>MTITPATHAISINPATGEQLSVLPWAGADDIENALQLAAAGFRDWRETNIDYRAEKLRDIGKALRARSEEMAQMITREMGKPINQARAEVAKSANLCDWYAEHGPAMLKAEPTLVENQQAVIEYRPLGTILAIMPWNFPLWQVMRGAVPIILAGNGYLLKHAPNVMGCAQLIAQVFKDAGIPQGVYGWLNADNDGVSQMIKDSRIAAVTVTGSVRAGAAIGAQAGAALKKCVLELGGSDPFIVLNDADLELAVKAAVAGRYQNTGQVCAAAKRFIIEEGIASAFTERFVAAAAALKMGDPRDEENALGPMARFDLRDELHHQVEKTLAQGARLLLGGEKMAGAGNYYPPTVLANVTPEMTAFREEMFGPVAAITIAKDAEHALELANDSEFGLSATIFTTDETQARQMAARLECGGVFINGYCASDARVAFGGVKKSGFGRELSHFGLHEFCNIQTVWKDRI[4x]

The NAD(P)+-dependent succinate semialdehyde dehydrogenase (SSADH) Sad is a member of the ALDH superfamily and oxidizes succinate semialdehyde (SSA) to succinate. In microorganisms, SSADHs operate in the degradation of various nitrogen-containing compounds such as putrescine or arginine, where they prevent the accumulation of the toxic SSA intermediate. Our results show that Sad is a surprisingly flexible enzyme that is not only able to detoxify succinate semialdehyde and glutarate semialdehyde but can also functionally substitute erythrose 4-phosphate dehydrogenase in pyridoxal 5′-phosphate (PLP) biosynthesis and glyceraldehyde 3-phosphate dehydrogenase (as well as phosphoglycerate kinase) in glycolysis under physiological conditions. We show that Sad, which primarily functions in the detoxification of succinate semialdehyde in various degradation pathways, does not only accept closely related substrates, but also converts phosphorylated sugars as a side reactivity.

To understand the molecular basis of the improved enzyme activity in the Q262R variant, we solved the crystal structures of both Sad WT and Q262R variants with bound NAD+, as well as in complex with both NAD+ and SSA. Even more surprisingly, when testing the substrate spectrum of Sad, we noticed that the WT enzyme was able to directly accept E4P, notably at four-fold higher activity (50 nmol min−1 mg−1) compared to D-erythrose. Moreover, in the Q262R variant, E4P dehydrogenase activity was increased 17-fold compared to the WT, reaching 800 nmol min−1 mg−1. Both variants were also active with glyceraldehyde 3-phosphate (GAP), showing even higher activities with GAP compared to E4P. GabD showed higher activity on SSA than any of the two Sad variants (164 ± 9 μmol min−1 mg−1) but was almost inactive with E4P and GAP, indicating that the promiscuity with phosphorylated C3 and C4 sugars was restricted to Sad. Compared to Sad WT, GabD only supported slow growth, likely due to its lower activity on E4P as well as the rather unfavorable intracellular NADP+/NADPH ratio to operate the oxidation reaction.> QCYHGNGQSYRGTF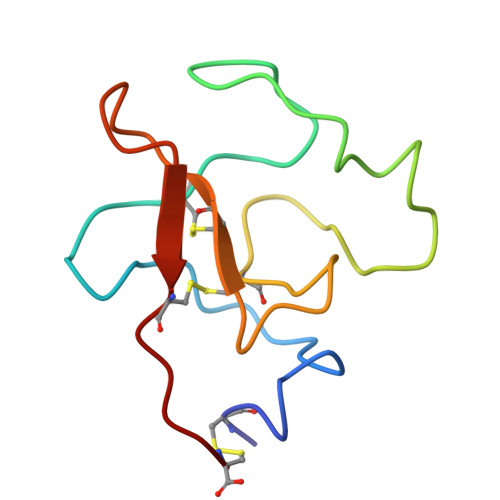STTVTGRTCQSWSSMTPHRHQRTPENYPNDGLTMNYCRNPDADTGPWCFTMDPSIRREYCNLTRC> GAGCAGACCTGA;> CGTCACTCA;> TCAACG;> TCTGAGTGGGTCTGC

In this work, we exhaustively probe the ability of all 36 immobile HJ sequences to form DNA crystals in two different designed systems. Three separate self-assembling DNA crystal systems are described in this report: the “4 × 5” and “4 × 6” designs (collectively referred to as the 4 × N systems), and a third construct with a “scrambled” sequence variant of the 4 × 6 lattices. Self-assembly was mediated by three constituent oligonucleotides: (S1) containing four sequence repeats of either 5 or 6 bases; (S2) composed of 21 bases containing complementary regions to both (S1); and (S3) which forms the second junction crossover. The HJ serves as the fundamental component at the core of each unit, and the ultimate assembly of the full lattice is facilitated by the complementary 2-base sticky ends that tail each duplex.

In parallel, we employed the previously reported J1 4 × 6 system (3.05 Å), with P32 symmetry. Seventeen of the 36 junctions successfully crystallized, a 47% success rate. Unlike the 4 × 5 motif, nearly all of the 4 × 6 junction sequences had a strong preference for crystallization in buffers containing ≥2.0 M salts (e.g., LiCl, Li2SO4, KCl, and NaCl), with the majority preferring slightly basic pH conditions in cacodylic acid. The average cell constants for the P32 crystals were a = b = 68.29 Å c = 55.68 Å.> MSGCRAQNAPGGIPVTPKSSYSGPIVVDPVTRIEGHLRIEVEVENGKVKNAYSSSTLFRGLEIILKGRDPRDAQHFTQRTCGVCTYTHALASTRCVDNAVGVHIPKNATYIRNLVLGAQYLHDHIVHFYHLHALDFVDVTAALKADPAKAAKVA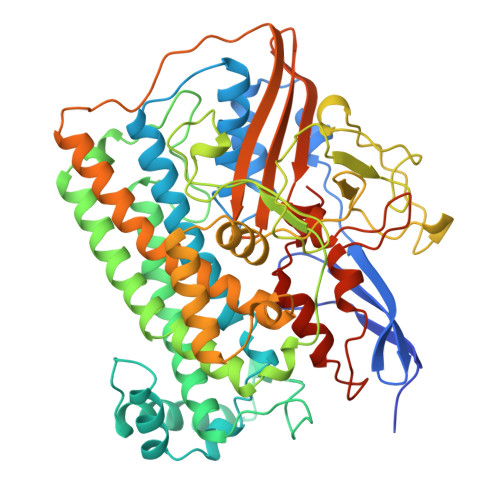SSISPRKTTAADLKAVQDKLKTFVETGQLGPFTNAYFLGGHPAYYLDPETNLIATAHYLEALRLQVKAARAMAVFGAKNPHTQFTVVGGVTCYDALTPQRIAEFEALWKETKAFVDEVYIPDLLVVAAAYKDWTQYGGTDNFITFGEFPKDEYDLNSRFFKPGVVFKRDFKNIKPFDKMQIEEHVRHSWYEGAEARHPWKGQTQPKYTDLHGDDRYSWMKAPRYMGEPMETGPLAQVLIAYSQGHPKVKAVTDAVLAKLGVGPEALFSTLGRTAARGIETAVIAEYVGVMLQEYKDNIAKGDNVICAPWEMPKQAEGVGFVNAPRGGLSHWIRIEDGKIGNFQLVVPSTWTLGPRCDKNNVSPVEASLIGTPVADAKRPVEILRTVHSFDPCIACGVHVIDGHTNEVHKFRIL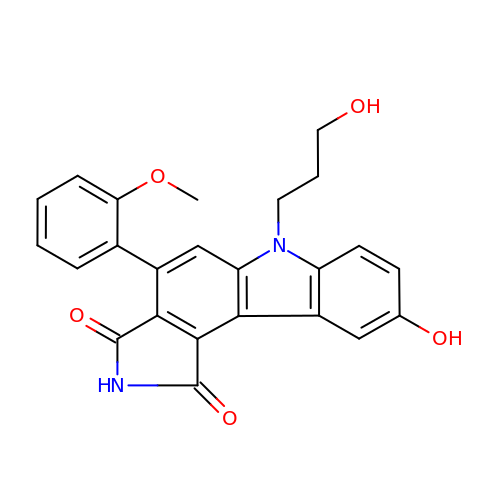9-HYDROXY-6-(3-HYDROXYPROPYL)-4-(2-METHOXYPHENYL)PYRROLO[3,4-C]CARBAZOLE-1,3(2H,6H)-DIONE | C24 H20 N2 O5 | AOGOZJCRIFBTTN-UHFFFAOYSA-N> 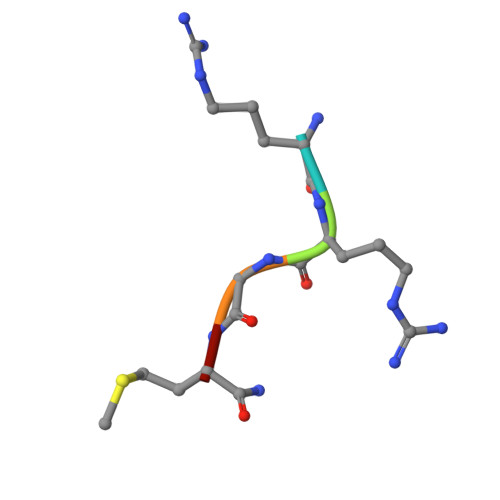RRGMX> EVEALRHDIQLDDDARVFVQANMDC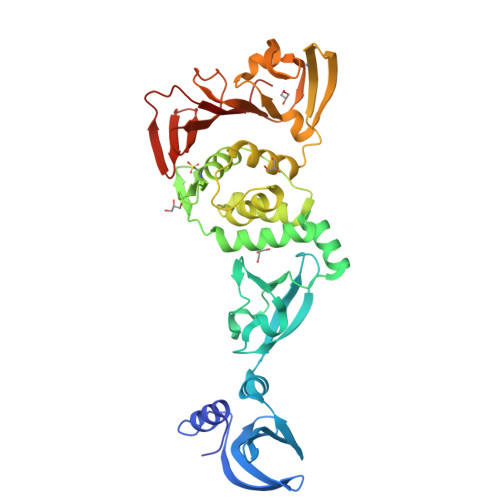LPTDWRLVNKFDSVDGVRTIKYFECPGGIFVSSQGKKFGYVQNGSFKEASVSQIRALLANKVDVLCTVDGVNFRSCCVAEGEVFGKTLGSVFCDGINVTKVRCSAIYKGKVFFQYSDLSEADLVAVKDAFGFDEPQLLKYYTMLGMCKWPVVVCGNYFAFKQSNNNCYINVACLMLQHLSLKFPKWQWQEAWNEFRSGKPLRFVSLVLAKGSFKFNEPSDSIDFMRVVLREADLSGATCNLEFVCKCGVKQEQRKGVDAVMHFGTLDKGDLVRGYNIACTCGSKLVHCTQFNVPFLICSNTPEGRKLPDDVVAANIFTGGSVGHYTHVKCKPKYQLYDACNVNKVSEAKGNFTDCLYLKNLK ANHYDRORETINOL | C20 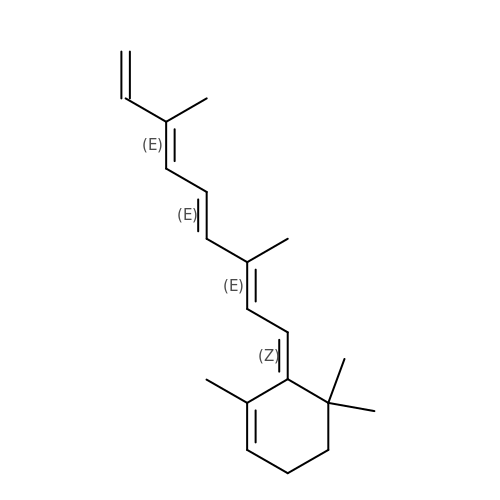H28 | FWNRILWHNGFAIN-OYUWDNMLSA-N>[2x]GQNH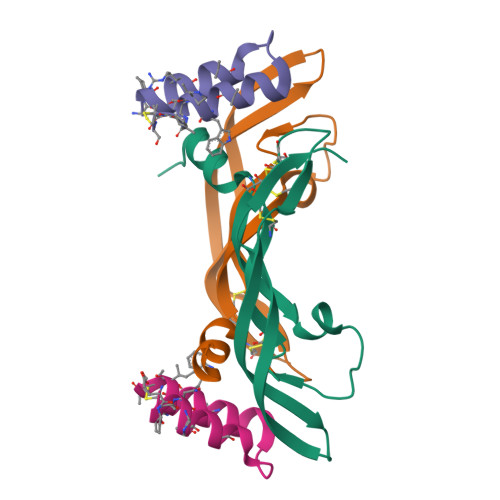HEVVKFMDVYQRSYCHPIETLVDIFQEYPDEIEYIFKPSCVPLMRCGGCCNDEGLECVPTEESNITMQIMRIKPHQGQHIGEMSFLQHNKCECRPKKD;>VDNKXNKEXCNXRAIEAALDPNLNDQQFHAKIWXIIXDCX[2x]>MHHHHHHHHENLYFQGSKEKFWKISTPPEAYWNREQEKLNRQYNPILSMLTNQTGEAGRLSNISHLNYCEPDLRVTSVVTGFNNLPDRFKDFLLYLRCRNYSLLIDQPDKCAKKPFLLLAIKSLTPHFARRQAIRESWGQESNAGNQTVVRVFLLGQTPPEDNHPDLSDMLKFESEKHQDILMWNYRDTFFNLSLKEVLFLRWVSTSCPDTEFVFKGDDDVFVNTHHILNYLNSLSKTKAKDLFIGDVIHNAGPHRDKKLKYYIPEVVYSGL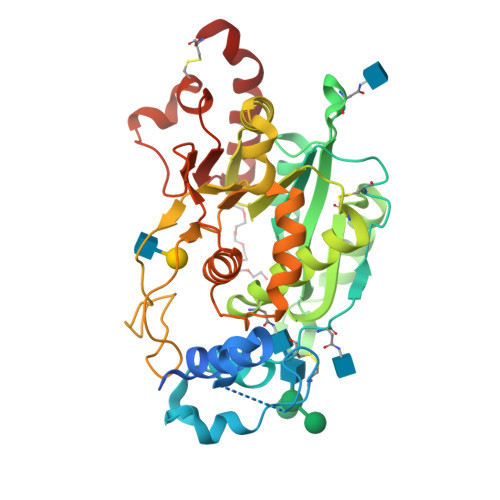YPPYAGGGGFLYSGHLALRLYHITDQVHLYPIDDVYTGMCLQKLGLVPEKHKGFRTFDIEEKNKNNICSYVDLMLVHSRKPQEMIDIWSQLQSAHLKC[2x]>KSSCKRHPLYVDFSDVGWNDWIVAPPGYHAFYCDGECSFPLNAHMNATNHAIVQTLVHLMNPEYVPKPCCAPTELS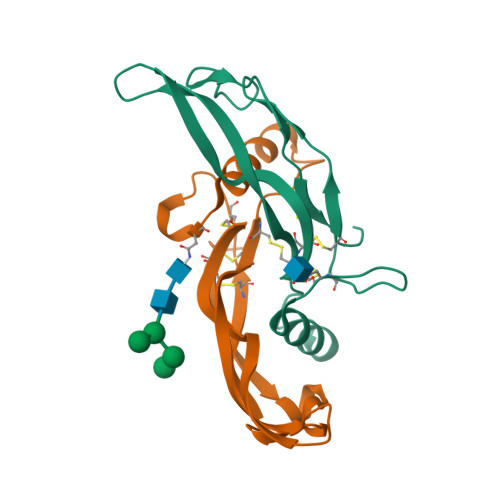AISMLYLDENEKVVLKNYQDMVVEGCGCR[2x]>[2x]MPNSEPASLLELFNSIATQGELVRSLKAGNASKDEIDSAVKMLVSLKMSYKAAAGEDYKADCPPGNPAPTSNHGPDATEAEEDFVDPWTVQTSSAKGIDYDKLIVRFGSSKIDKELINRIERATGQRPHHFLRR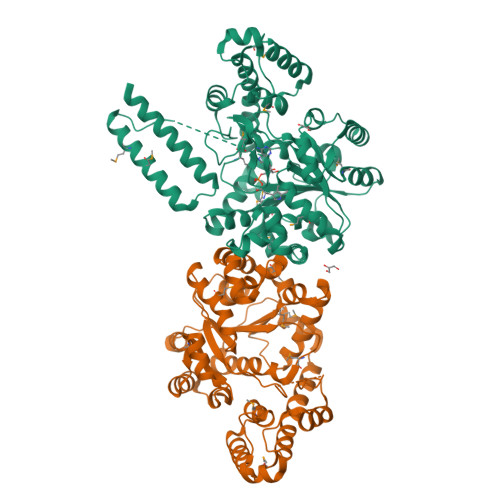GIFFSHRDMNQVLDAYENKKPFYLYTGRGPSSEAMHVGHLIPFIFTKWLQDVFNVPLVIQMTDDEKYLWKDLTLDQAYGDAVENAKDIIACGFDINKTFIFSDLDYMGMSSGFYKNVVKIQKHVTFNQVKGIFGFTDSDCIGKISFPAIQAAPSFSNSFPQIFRDRTDIQCLIPCAIDQDPYFRMTRDVAPRIGYPKPALLHSTFFPALQGAQTKMSASDPNSSIFLTDTAKQIKTKVNKHAFSGGRDTIEEHRQFGGNCDVDVSFMYLTFFLEDDDKLEQIRKDYTSGAMLTGELKKALIEVLQPLIAEHQARRKEVTDEIVKEFMTPRKLAAALEHHHHHH> LGTNYLLSGQTLETEGHLKNGDFDLVMQDDCNLVLYNGNWQSNTANKGRDCKLTLTDYGELVINNGDGSTVWRSKAQSVKGDYAAVDHPE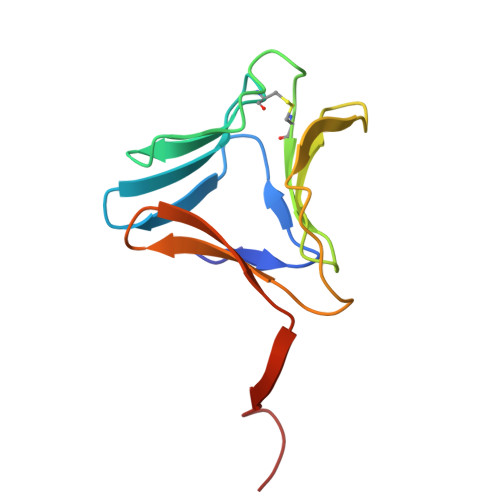GRLVVFGPSVFKIDPWVPG>[2x]GDPAERTWIFSGAELKQAIEGKLAPDVSDPEMRRLVSVAKSSAYIAGVADLTSGSDWCGAGAVAPHELTDRIYTYLGDMPAEKLDEQAATLVREALKVSFPCEQKSN;>[2x]MMRVNFDTLYSNYPSSDPSHPNYLSQRDLFTEIGWE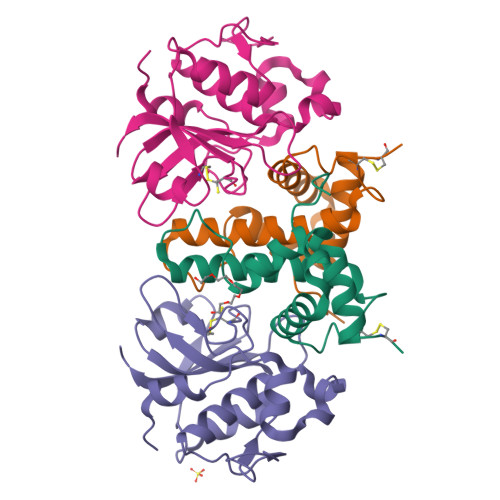SFIGNPNYHNTCAIRVSIAFVKSGINIVPSSHRIQKGPYAGKGIEVNMRRLATLMKRTSYLGEPDPYTPATARNGIGARNGVVAFNNIPGYTGGGHIDLVRGGSEATQCASACYYNSETIWFWPLQAS>MRCIGISNRDFVEGVSGGSWVDIVLEHGSCVTTMAKNKPTLDFELIKTEAKQPATLRKYCIEAKLTNTTTESRCPTQGEPSLNEEQDKRFVCKHSMVDRGWGNGCGLFGKGGIVTCAMFRCKKNMEGKVVQPENLEYTVVITPHSGEEHAVGNDTGKHGKEVKITPQSSITEAELTGYGTVTMECSPRTGLDFNEMVLLQMENKAWLVHRQWFLDLPLPWLPGADTQGSNWIQKETLVTFKNPHAKKQDVVVLGSQEGAMHTALTGATEIQMSSGNLLFTGHLKCRLRMDKLQLKGMSYSMCTGKFKVVKEIAETQHGTIVIRVQYEGDGSPCKIPFEIMDLEKRHVLGRLITVNPIVTEKDSPVNIEAEPPFGDSYIIIGVEPGQLKLDWFKKG[3x];>FHLTTRNGEPHMIVSRQEKGKSLLFKTE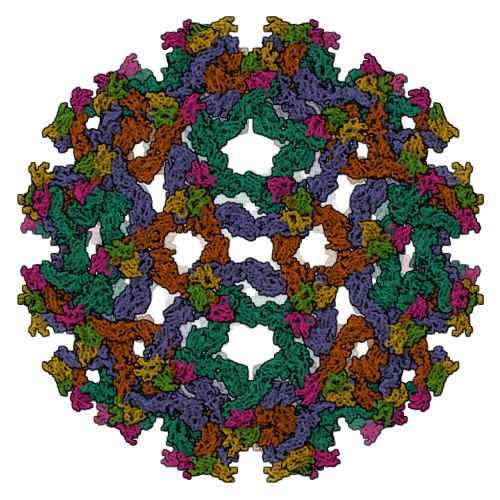DGVNMCTLMAMDLGELCEDTITYKCPLLRQNEPEDIDCWCNSTSTWVTYGTCT[3x]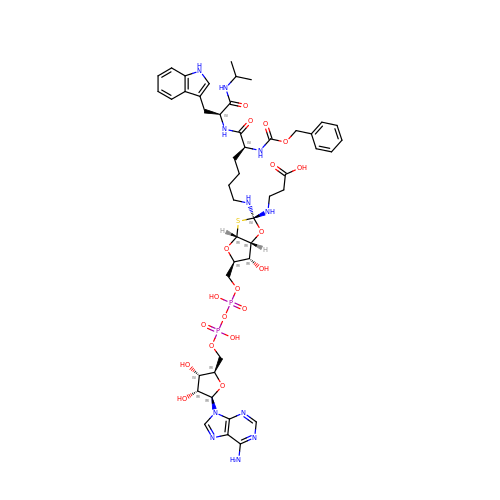3-[[(2~{S},3~{a}~{R},5~{R},6~{R},6~{a}~{R})-5-[[[[(2~{R},3~{S},4~{R},5~{R})-5-(6-aminopurin-9-yl)-3,4-bis(oxidanyl)oxolan-2-yl]methoxy-oxidanyl-phosphoryl]oxy-oxidanyl-phosphoryl]oxymethyl]-2-[[(5~{S})-6-[[(2~{S})-3-(1~{H}-indol-3-yl)-1-oxidanylidene-1-(propan-2-ylamino)propan-2-yl]amino]-6-oxidanylidene-5-(phenylmethoxycarbonylamino)hexyl]amino]-6-oxidanyl-3~{a},5,6,6~{a}-tetrahydrofuro[2,3-d][1,3]oxathiol-2-yl]amino]propanoic acid | C47 H63 N11 O19 P2 S | YXTVLLWQDXVSFE-WDVUSYHVSA-N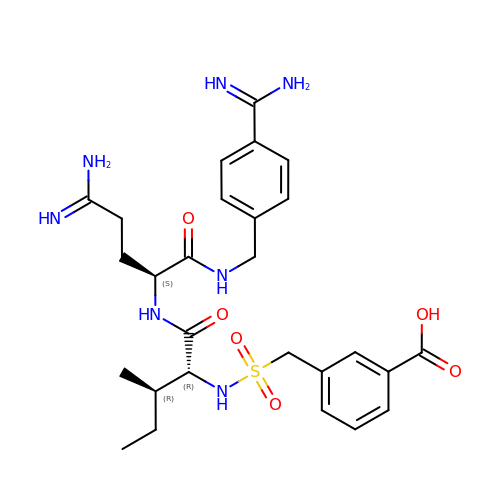N-[(3-CARBOXYBENZYL)SULFONYL]ISOLEUCYL-N~1~-{4-[AMINO(IMINO)METHYL]BENZYL}-5-IMINOORNITHINAMIDE | C27 H37 N7 O6 S | UBGNMISWPGURDN-XORNHQRDSA-N>[3x]DDYSFSCYSQLEVNGSQHSLTCAFEDPDVNITNLEFEICGALVEVKCLNFRKLQEIYFIETKKFLLIGKSNICVKVGEKSLTCKKIDLTTIVKPEAPF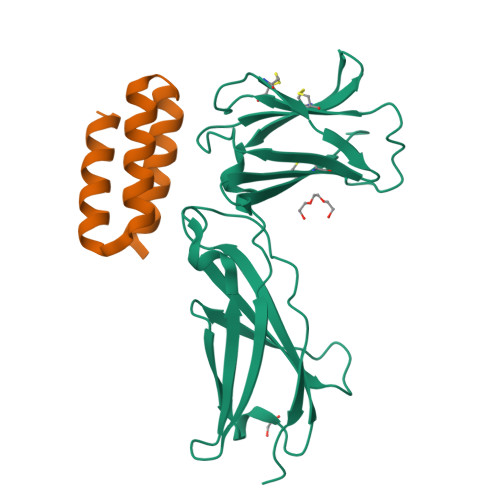DLSVVYREGANDFVVTFNTSHLQKKYVKVLMHDVAYRQEKDENKWTHVNLSSTKLTLLQRKLQPAAMYEIKVRSIPDHYFKGFWSEWSPSYYFRTPEI;>[3x]SVIEKLRKLEKQARKQGDEVLVMLARMVLEYLEKGWVSEEDADESADRIEEVLKK> MKRIKCNKVRTVTEIVNSDEKIQKTYELAEFDLKNLSSLESYETLKIKLALSKYMAMLSTLEMTQPLLEIFRNKADTRQIAAVVFSTLAFIHNRFHPLVTNFTNKMEFVVTETNDTSIPGEPILFTENEGVLLCSVDRPSIVKMLSREFDTEALVNFENDNCNVRIAKTFGASKRKNTTRSDDYESNKQPNYDMDLSDFSIT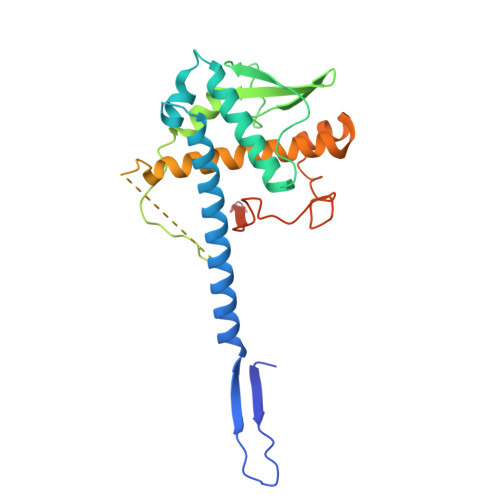EVEATQYLTLLLTVEHAYLHYYIFKNYGVFEYCKSLTDHSLFTNKLRSTMSTKTSNLLLSKFKFTIEDFDKINSNSVTSGFNIYNFNK> DNFQDLFTGAYHKYKVWRRQQMSFINKHERTLAIDGDYIYIVPPEGRIHWHDNVKTKSLHISQVVLVKKSKRVPEHFKIFVRREGQDDIKRYYFEAVSGQECTEIVTRL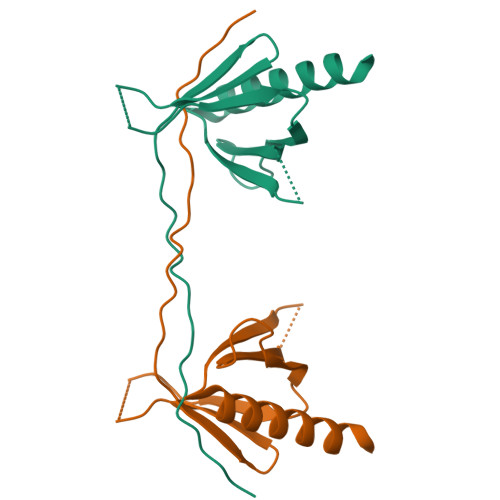QNLLSAYRMNHK>MNQETLIAVVEQMRKLVPALRKVPDETLYAWVEMAELFVCQKTFKDAYVKALALYALHLAFLDGALKGEDEDLESYSRRVTSFSLSGEFSQTFGEVTKNQSGDMMLSTPWGKMFEQLKARRRGRFALMTGLRGGCH[12x];>[12x]MKIVKHDGYNDIFNGGADGSPKPFFMSDASYHVGSFYNDNATAKRIVDVIPEEMVTAGFKMSGVKDEKEFKSLWDSYKLDSSLVDLLCWARLYGGAAMVAIIKDNRMLTSQAKPGAKLEGVRVYDRFAITVEKRVTNARSPRYGEPEIYKVSPGDNMQPYLIHHSRVFIADGERVAQQARKQNQGWGASVLNKSLIDAICDYDYCESLATQILRRKQQAVWKVKGLAEMCDDDDAQYAARLRLAQVDDNSGVGRAIGIDAETEEYDVLNSDISGVPEFLSSKMDRIVSLSGIHEIIIKNKNVGGVSASQNTALETFYKLVDRKREEDYRPLLEFLLPFIVDEEEWSIEFEPLSVPSKKEESEITKNNVESVTKAITEQIIDLEEARDTLRSIAPEFKLKDGNNINIREPEETTEPEPGLGE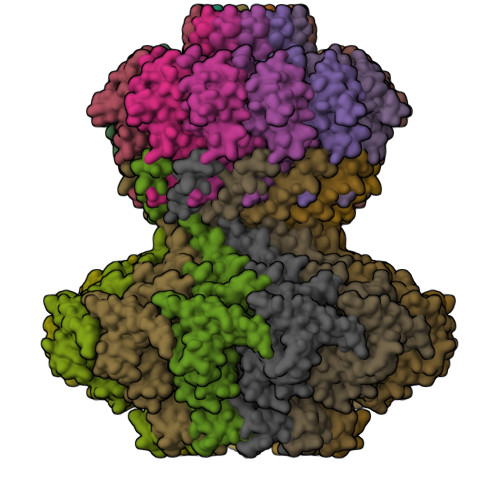KLEDEN> MSAANADFELFRVFLEKTCGIVLGSNKQYLVSSRLNKLMEQQGIKSLGELVQRIQTQRGGLREMVVDAMTTNETLWFRDTYPFEVLKQRVLPELIKANGGQRLRIWSAACSSGQEPYSLSMAIDEFEKTNLGQLKAGVQIVATDLSGSMLTAAKAGEYDTLAMGRGLSPERLQR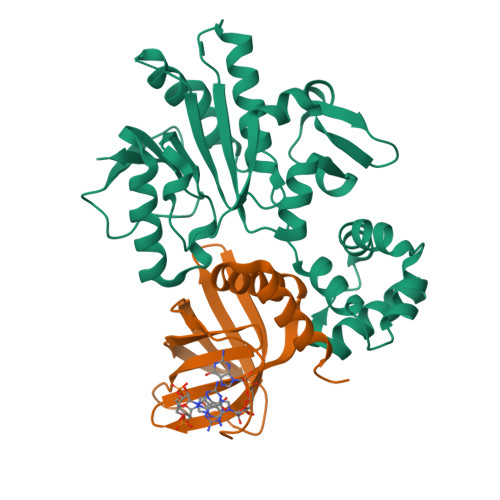YFDAKGPGRWAVKPAIRSRVEFRALNLLDSYASLGKFDMVFCRNVLIYFSAEVKRDILLRIHGTLKPGGYLFLGASEALNNLPDHYQMVQCSPGIIYRAKLEHHHHH;> MSDQHDERRRFHRIAFDADSEILQGERRWEVLLHDVSLHGILVGQPQDWNGDPQRPFEARLYLGLDVLIRMEISLAWARDGLLGFECQHIDLDSISHLRRLVELNLGDEELLERELALLVSAHDDLEHHHHHH> NAVESTLRRVAKDLTGLRQRWALVGGFAVSARSEPRFTRDVDIVVAVANDDAAESLVRQLLTQQYHLLASVEQDAARRLAAVRLGATADTAANVVVDLLFASCGIEPEIAEAAEEIEILPDLVAPVATTAHLIAMKLLARDDDRRPQDRSDLRALVDAASPQDIQDARKAIELITLRGFHRDRDLAAEWTRLAAKW

The Mycobacterium tuberculosis NTase toxin family, MenT, modifies tRNAs to block translation. MenT toxin activity can be stringently regulated by diverse MenA antitoxins. MenT and AbiEii toxins share four highly conserved NTase motifs scattered throughout their structures, proposed to facilitate co-ordination of metals (motifs I and II), base stacking, and transfer of nucleotides to tRNA isoacceptors (motif III), and to contribute to catalysis (motif IV). Our study reveals a conserved mechanism for the control of tuberculosis toxins, and demonstrates how active site auto-phosphorylation can regulate the activity of widespread NTases.

Here we demonstrate through structural, biochemical, biophysical and computational studies that despite lacking kinase motifs, antitoxin MenA1 induces auto-phosphorylation of MenT1 by repositioning the MenT1 phosphoacceptor T39 active site residue towards bound nucleotide. We analysed the MenAT1 co-expression sample by Liquid Chromatography Tandem Mass Spectrometry (LC-MS/MS), which confirmed that T39 is the site of MenT1 phosphorylation. The MenT1-p structure shows clear density for a phosphothreonine (TPO) at position T39. Alignment of each structure via C-alpha atoms only returned an RMSD of 0.410 Å (160 atoms), indicating a near identical topology of core domains and folds. In contrast, aligning the C-alpha atoms of the respective T39 loops returned an RMSD of 0.778 Å (7 atoms), indicating a larger shift between these specific loops. Close-up views revealed further changes caused by the presence of the phosphothreonine, such as steric occlusion of the active site. Structural alignments also revealed that residues R37 and F38 are both ejected from the toxin active site following phosphorylation. However, phosphorylation greatly reduces the net positive charge within the MenT1 active site. Accordingly, when MenT1 and MenT1-p were incubated with E. coli tRNAs from the cell-free PURExpress translation system, we found that MenT1-p was unable to inhibit GFP protein synthesis. When compared against the calculated Rst of this model, the observed Rst of the unknown species almost perfectly matches that of the hypothetical heterodimer, returning an observed/calculated Rst ratio of 0.97. These data suggest that MenT1-p can form a stable heterodimer, but not a heterotrimeric complex.> MFGSGNVLPVKIQPPLLRPLAYRVLSRKYGLSIKSDGLSALAEFVGTNIGANWRQGPATIKFLEQFAAVWKQQERGLFIDQSGVKEVIQEMKEREKVEWSHEHPIQHEENILGRTDDDENNSDDEMPIAADSSLQNVSLSSPMRQPTERDEYKQPFKPESSKALDWRDYFKVINASQQQRFSYNPHKMQFIFVPNKKQNGLGGIAGFLPDIEDKVQMFLTRYYLTNDRVMRNENFQNSDMFNPLSSMVSLQNELSNTNRQQQSSSNSITPIKNLLGRDAQNFLLLGLLNKNFKGNWSLEDPSGSVEIDISQTIPTQGHYYVPGCMVLVEGIYYSVGNKFHVTSMTLPPGERREITLETIGNLDLLGIHGISNNNFIARLDKDLKIRLHLLEKELTDHKFVILGANLFLDDLKIMTALSKILQKLNDDPPT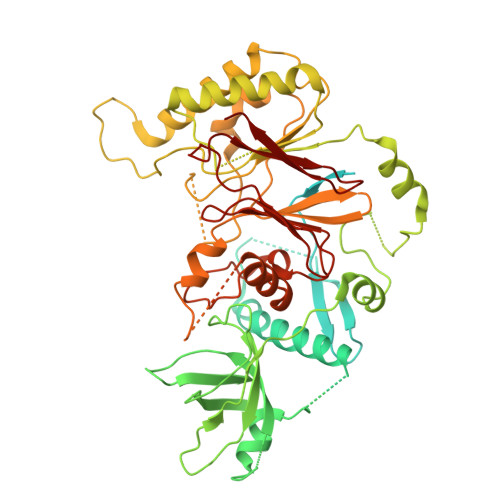LLIWQGSFTSVPVFASMSSRNISSSTQFKNNFDALATLLSRFDNLTENTTMIFIPGPNDLWGSMVSLGASGTLPQDPIPSAFTKKINKVCKNVVWSSNPTRIAYLSQEIVIFRDDLSGRFKRHRLEFPFNESEDVYTENDNMMSKDTDIVPIDELVKEPDQLPQKVQETRKLVKTILDQGHLSPFLDSLRPISWDLDHTLTLCPIPSTMVLCDTTSAQFDLTYNGCKVINPGSFIHNRRARYMEYVPSSKKTIQEEIYI>[2x]MHQDYRELSLDELESVEKQTLRTIVQALQQYSKEAKSIFETTAADSSGEVIVLAEDITQYALEVAETYPINRRFAGFIDYKRVRWLPSPHGLLPQVLLVDAKASTEKNRD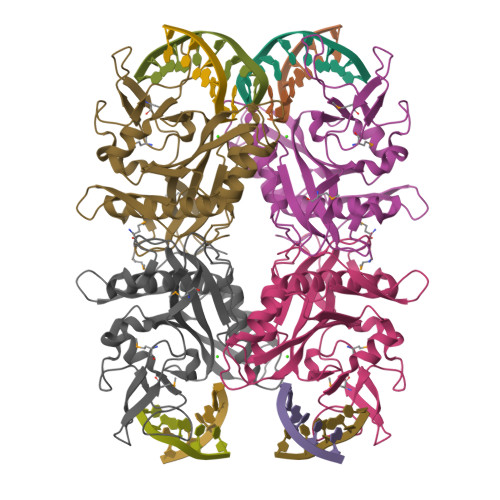TLQRSQLPMDAEFRNTSSGEVVTMEAGVIPHLMLQSANDGVLPAVTTSIFVHFYYRELKDVEGRYRELKSIYVLSLPHARLKQRYNPDPDTSFFGAGKHSPARGEVARIRVYFDRLKEACPWRLQELHYSADSEYTQPRWRDLNDAGHEVTKEFLFLER> GSTRYVPYTIAVNGTSTPILSKLKISNKQLISYKYLNDKVKSVLKSERGISDLDLKFAKQAKYTVYFKNGKKQVVNLKSDIFTPNLFS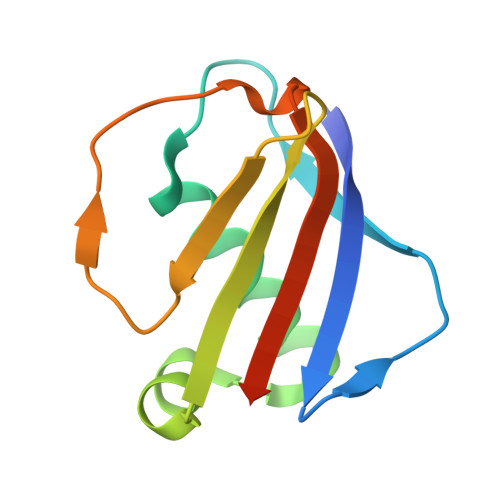AKDIKKIDIDVKQYTKSKKK>[10x]MRIYSRLFQISSANYARQIMSNQFIKAKESKGLTYQQMAQLLSVNKVWLTSVLHGQNCCDIQLAHRICDTLGISHEYANELTSIPLRGNQNIINDPLIYRFNELFKVYGSSLR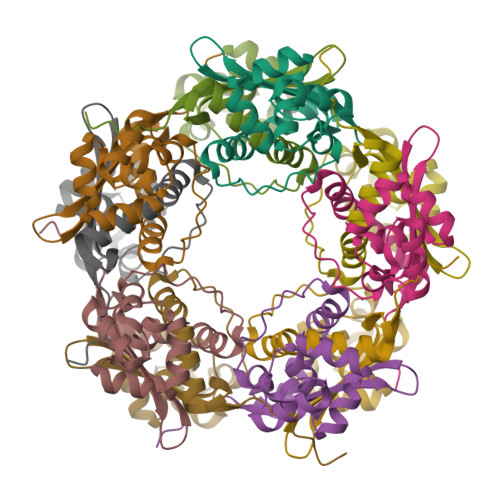GIIHEEFGDGIMSAIDCKIDVTKNEQSRVILRIDGKFLPYYKGQLDAGENLYFQSAGHHHHHH[4-[3-(4-bromophenyl)-3-oxidanylidene-propyl]-6-methyl-5-oxidanyl-pyridin-3-yl]methyl 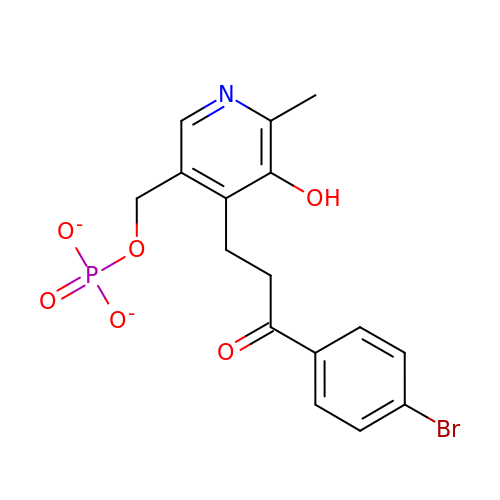phosphate | C16 H15 Br N O6 P | LURUZQWETZCIOP-UHFFFAOYSA-L> SSVTADLNNAVINVDEMNEAFKDVPDLEGEGAHITLSNTTAKPGEMAEVTMSVSNADMQWNMCGIHIIYPDILKPEMKDPEERTVAFQKGDALEAATGIVCMEWQEGLPPVLTENKKGCLFLTAMFSGNQGGEGDMATFR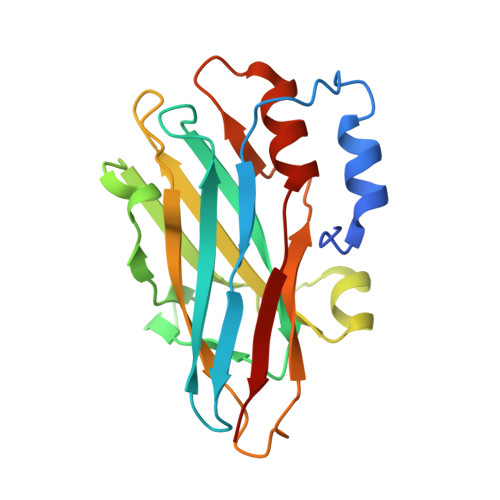FKVPDNAEPGAVYNLGYYYMNTDLFINEQNIPTYQKYAFTHMEGGTITVEL> GPLGSPEFMINGVSLQGTAGYEAHTEEGNVNVKKLLESLNSKSLGDMDKDSELAATLQKMINPSGGDGNASGCALHACMAMLGYGVREAPVPNEISEYMTGFFHRHLEQIDSEGIVSHPNETYSKFRERIAENILQNTSKGSVVMISIEQATHWIAGFNDGEKIMFLDVQTGKGFNLYDPVEKSPDAFVDENSSVQVIHVSDQEFDHYANSSSWKSKRLC;> GSHMAGLPRRIIKETQRLLAEPVPGIKAEPDESNARYFHVVIAGPQDSPFEGGTFKLELFLPEEYPMAAPKVRFMTKIYHPNVDKLGRICLDILKDKWSPALQIRTVLLSIQALLSAPNPDDPLAN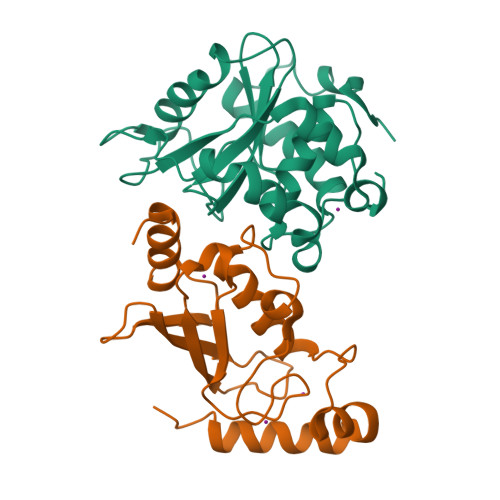DVAEQWKTNEAQAIETARAWTRLYAMNNI N-(3-chlorophenyl)-6,7-dimethoxyquinazolin-4-amine 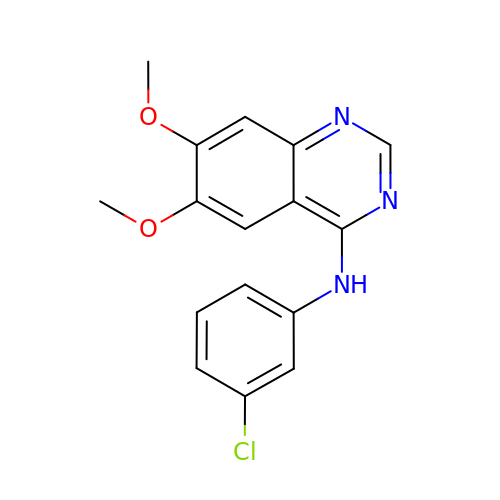| C16 H14 Cl N3 O2 | GFNNBHLJANVSQV-UHFFFAOYSA-N>SVIKPDMKIKLRMEGAVNGHPFAIEGVGLGKPFEGKQSMDLKVKEGGPLPFAYDILTMAFCYGNRVFAKYPENIVDYFKQSFPEGYSWERSMIYEDGGICNATNDITLDGDCYIYEIRFDGVNFPANGPVMQKRTVKW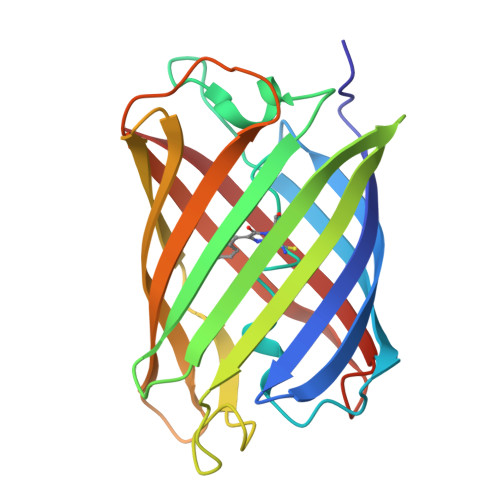ELSTEKLYVRDGVLKSDGNYALSLEGGGHYRCDFKTTYKAKKVVQLPDYHSVDHHIEIKSHDKDYSNVNLHEHAEAHS[6x]>[2x]MAHHHHHHMIQVGDALPDAQLFEFIDDAREGCTLGPNACSVRDQVAGKRVVIFGLPGAFTPTCSAQHVPGYVEHAEQLRAAGIDEIWCVSVNDAFVMGAWGRDLHTAGKVRMMAD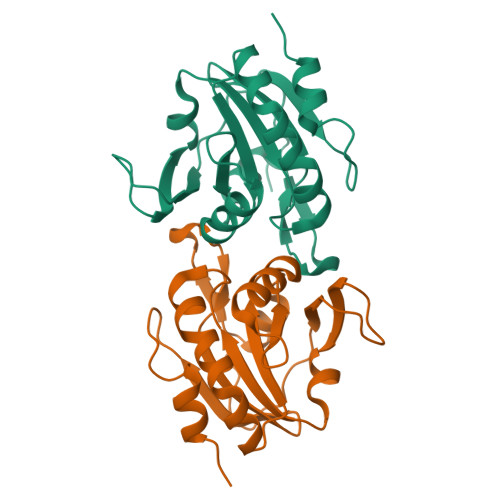GSAAFTHALGLTQDLSARGMGIRSLRYAMVIDGGVVKTLAVEAPGKFEVSDAASVLATLTS>MEHHHHHHATNLRGVMAALLTPFDQQQALDKASLRRLVQFNIQQGIDGLYVGGSTGEAFVQSLSEREQVLEIVAEEAKGKIKLIAHVGCVSTAESQQLAASAKRYGFDAVSAVTPFYYPFSFEEHCDHYRAIIDSADGLPMVVYNIPALSGVKLTLDQINTLVTLPGVGALKQTSGDLYQMEQIRREHPDLVLYNGYDEIFASGLLAGADGGIGSTYNIMGWRYQGIVKALKEGDIQTAQKLQTECNKVIDLLIKTGVFRGLKTVLHYMDVVSVPLCRKPFGPVDEKYLPELKALAQQLMQER[4x]

N-Acetylneuraminic acid lyase (NAL; EC 4.1.3.3, otherwise known as N-acetylneuraminic acid aldolase or sialic acid aldolase) catalyzes the reversible aldol condensation of N-acetylmannosamine (ManNAc) with pyruvate to yield the most abundant sialic acid N-acetylneuraminic acid (Neu5Ac). Sialic acids are essential components of complex carbohydrates that play pivotal roles as recognition signals in a variety of biological processes. The residue responsible for this alteration of specificity at position 192 lies at one end of the active-site cleft opposite the active-site catalytic residue Lys165, which forms a Schiff base with the substrate as part of the catalytic cycle. In order to probe the mechanism by which alteration of the residue at position 192 affects substrate specificity, we have undertaken an analysis of the activity of all 20 variants of NAL at position 192 along with an X-ray structural analysis of the E192N enzyme in the absence and in the presence of a competitive inhibitor, (2R,3R)-2,3,4-trihydroxy-N,N-dipropylbutanamide (THB).

We therefore identified new conditions for the crystallization of E. coli NAL (in space group P21) that avoided the use of sulfate ions and allowed us to solve the structures of both the wild type and the E192N variant in the presence and in the absence of a number of ligands. The structures of complexes with pyruvate were also obtained (to 1.65 Å resolution for the wild-type enzyme and to 1.8 Å resolution for E192N). As expected, pyruvate was covalently linked to Lys165, and the planarity of electron density is consistent with the formation of the natural pyruvate enamine intermediate. The interactions made by pyruvate in that structure and in the P21 structures of the wild-type–pyruvate and E192N–pyruvate complexes reported here are identical. Comparison with the apo-NAL structures indicates that there are no significant changes in the active site upon pyruvate binding; the only difference in the two structures appears to be a further disordering of the C-terminal residues in a remote location from the catalytic pocket.>MEEVFQNETIKQILAKYRRIWAIGHAQSVLGWDLEVNMPKEGILERSVAQGELSVLSHELLLHPEFVNLVEKAKGLENLNEYERGIVRVLDRSIRIARAFPPEFIREVSETTSLATKAWEEAKAKDDFSKFEPWLDKIISLAKRAAEYLGYEEEPYDALLDLYEEGLRTRDVEKMFEVLEKKLKPLLDKILEEGKVPREHPLEKEKYEREWMERVNLWILQKFGFPLGTRARLDVSAHPFTTEFGIRDVRITTRYEGYDFRRTILSTVHEFGHALYELQQDERFMFTPIAGGVSLGIHESQSRFWENIIGRSKEFVELIYPVLKENLPFMSNYTPEDVYLYFNIVRPDFIRTEADVVTYNFHILLRFKLERLMVSEEIKAKDLPEMWNDEMERLLGIRPRKYSEGILQDIHWAHGSIGYFPTYTIGTLLSAQLYYHIKKDIPDFEEKVAKAEFDPIKAWLREKIHRWGSIYPPKE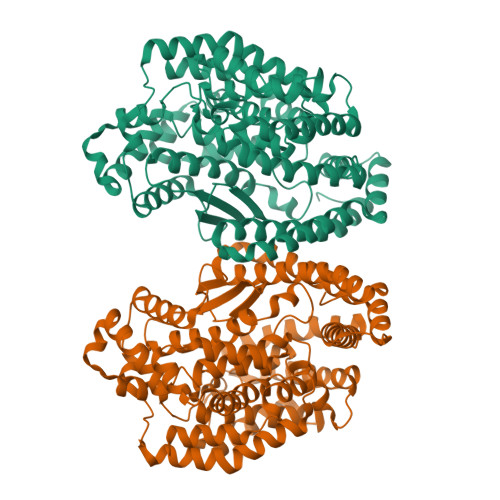LLKKAIGEDMDAEYFVRWVKEKYL[4x]> LPTSNPAQELEARQLERTTRDDLINGNSASCADVIFIYARGSTETGNLGTLGPSIASNLESAFGKDGVWIQGVGGAYRATLGDNALPRGTSSAAIREMLGLF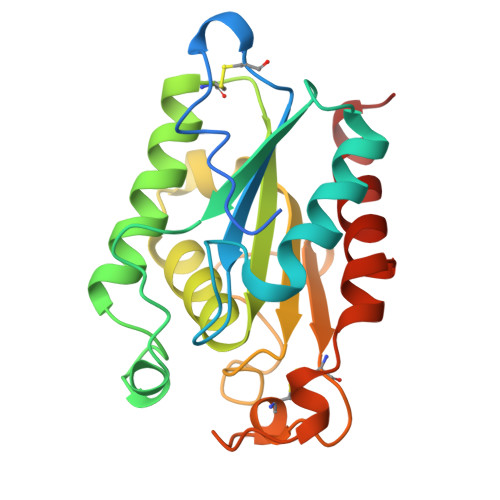QQANTKCPDATLIAGGYSQGAALAAACIEDLDSAIRDKIAGTVLFGYTKNLQNRGRIPNYPADRTKVFCNTGDLVCTGSLIVAAPHLAYGPDARGPAPEFLIEKVRAVRGSA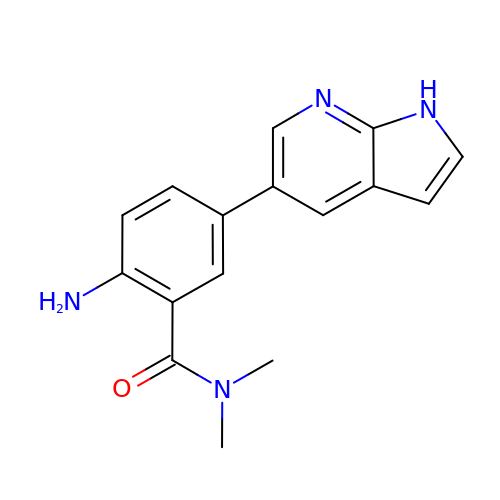2-amino-N,N-dimethyl-5-(1H-pyrrolo[2,3-b]pyridin-5-yl)benzamide | C16 H16 N4 O | NYTIYMREXUPYRJ-UHFFFAOYSA-N>[2x]GSMVTAPLRIDRAGRVQTWTIDVPDAANAITGSDFIDAFDAAVDAANADTDISVVILTGAGRFFSAGGNVRDMRDRTGVFGLGPLDQRHGYSSGIQRVPRALQRCEVPVIAAVNGAAIGAGCDLAVMCDLRIAAESAFFAESFVQLGLIPGDGGTWFLPRAVGWAR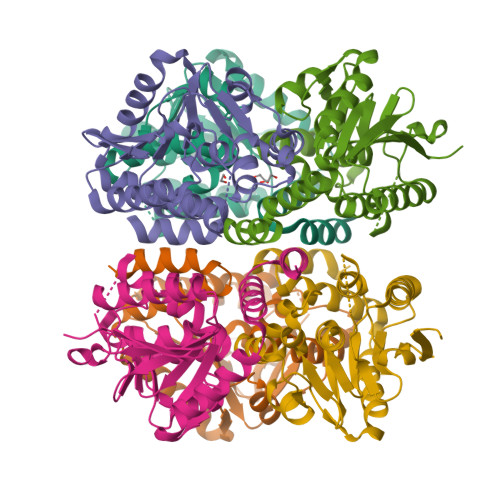AAEMTLTGDRVDAATALSWGLVNEVLSDDELLPAAHRLAERIAKNPAPAVRMAKRLLLESRTASLDSTLALAAALQPLAHQDPEHHRRVAELTR>GPLAPYEIIVSEDSEHLGKSIGELNVWHQTGATIVAIEHEGKFIVSP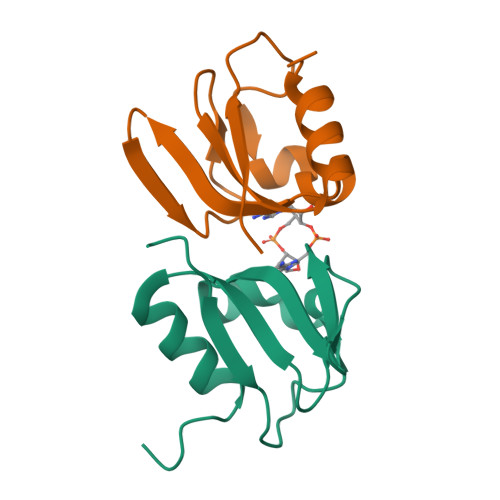GPFSVIEQGDHIFFVGDEDVYARMKTYFNLRMGL[2x]> MHNHNHN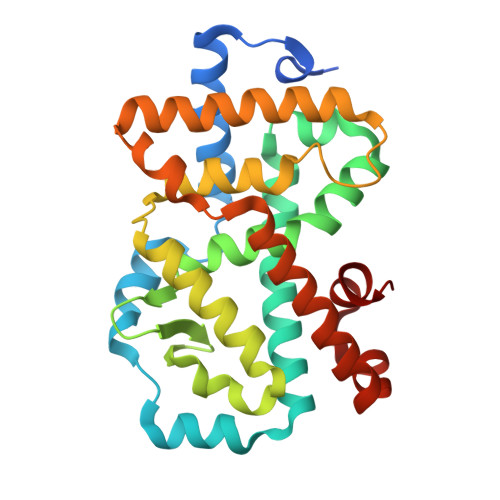HNHNHNGGENLYFQGASLTEIEHLVQSVCKSYRETCQLRLEDLLRQRSNIFSREEVTGYQRKSMWEMWERCAHHLTEAIQYVVEFAKRLSGFMELCQNDQIVLLKAGAMEVVLVRMCRAYNADNRTVFFEGKYGGMELFRALGCSELISSIFDFSHSLSALHFSEDEIALYTALVLINAHRPGLQEKRKVEQLQYNLELAFHHHLCKTHRQSILAKLPPKGKLRSLCSQHVERLQIFQHLHPIVVQAAFPPLYKELFSGG>MFDFIIDFETMGSGEKAAVIDLAVIAFDPNPEVVETFDELVSRGIKIKFDLKSQKGHRLFTKSTIEWWKNQSPEARKNIAPSDEDVATIAGIAKFNDYINAHNIDPWKSQGWCRGMSFDFPILVDLIRDIQRLNGVSENELDTFKLEPCKFWNQRDIRTRIEALLLVRDMT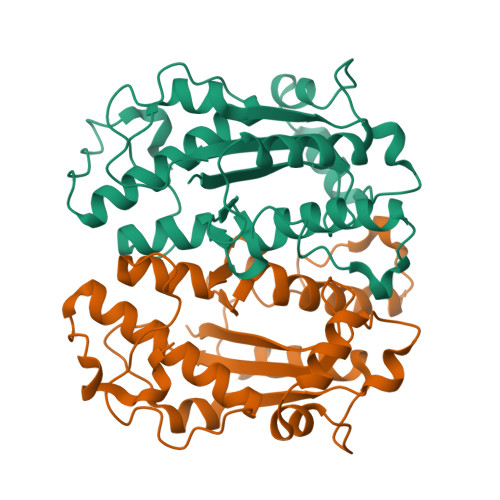TCPLPKGTLDGFVAHDSIHDCAKDILMMKYALRYAMGLEDAPSEEECDPLSLPTKR[2x]4-deoxy-L-erythro-hex-5-ulosuronic acid | C6 H8 O6 | 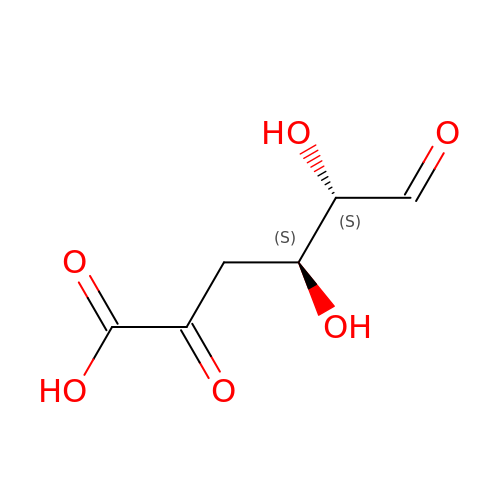IMUGYKFHMJLTOU-WVZVXSGGSA-N> MEQKTLQVEGMSCQHCVKAVETSVG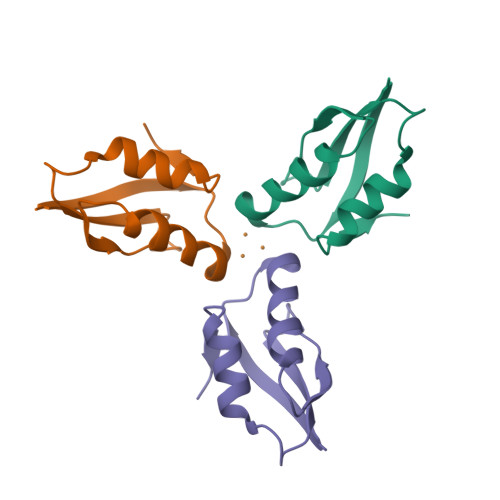ELDGVSAVHVNLEAGKVDVSFDADKVSVKDIADAIEDQGYDVAK>[3x]GSHMSKKILIVESDTALSATLRSALEGRGFTVDETTDGKGSVEQIRRDRPDLVVLA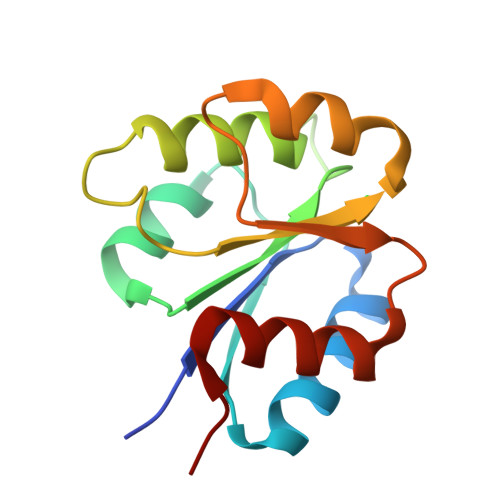VDLSAGQNGYLICGKLKKDDDLKNVPIVIIGNPDGFAQHRKLKAHADEYVAKPVDADQLVERAGALIGFPE> MTNDNSGIWVLGYGSLIYKPPSHYTHRIPAIIHGFARRFWQMSTDHRGTPANPGRVATLIPYEDIIRQTAFLKNVNMYSESAPIQDPDDLVTIGVVYYIPPEHAQEVREYLNVREQNGYTLHEVEVHLETNREHEAELGEMLEQLPRHNKSG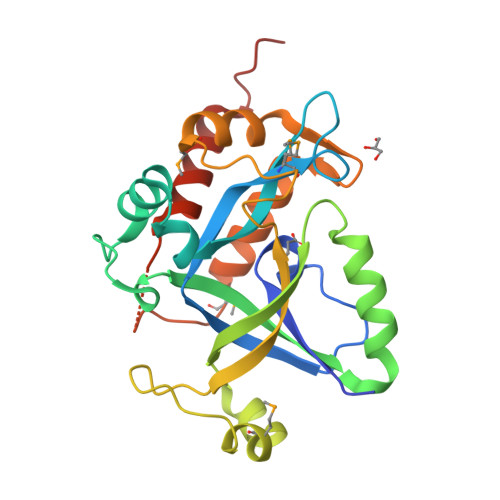KRVLLTSVYIGTIDNEAFVGPETMDETAKVIAVSHGPSGSNYEYLAKLEQALAQMPIMKERGRITDHYLTALLETVNKYRHHHHHHHH>[2x]MAHHHHHHGSMPISKIHARSVYDSRGNPTVEVDVVTETGLHRAIVPSGASTGQHEAHELRDGDKTQWGGKGVLKAVKNVNET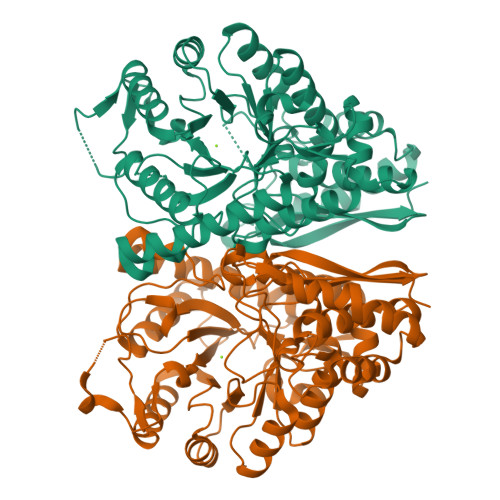IGPALIKENIDVKDQSKVDEFLNKLDGTANKSNLGANAILGVSLAVAKAGAAEKGVPLYAHISDLAGTKKPYVLPVPFQNVLNGGSHAGGRLAFQEFMIVPDSAPSFSEALRQGAEVYQKLKALAKKKYGQSAGNVGDEGGVAPDIQTAEEALDLITEAIEQAGYTGKIKIAMDVASSEFYKADVKKYDLDFKNPESDPSKWLTYEQLADLYKSLAAKYPIVSIEDPFAEDDWEAWSYFYKTSDFQIVGDDLTVTNPGRIKKAIELKSCNALLLKVNQIGTLTESIQAAKDSYADNWGVMVSHRSGETEDVTIADIAVGLRSGQIKTGAPCRSERLAKLNQILRIEEELGENAVYAGSKFRTAVNL>GNSGRFERDAFDTLFDHAPDKLSVVKKSLITFVNKHLNKLNLEVTELETQFADGVYLVLLMGLLEDYFVPLHHFYLTPESFDQKVHNVSFAFELMLDGGLKKPKARPEDVVNLDLKST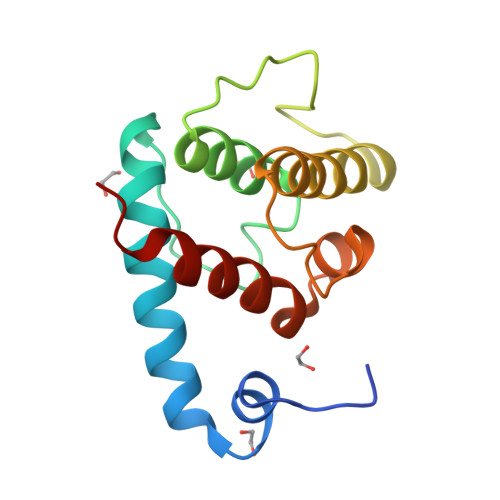LRVLYNLFTKYKNVE[6x]(2~{R},4~{S})-2-[(1~{R})-2-(azepan-1-yl)-1-formamido-2-oxidanylidene-ethyl]-5,5-dimethyl-1,3-thiazolidine-4-carboxylic acid | C15 H25 N3 O4 S | 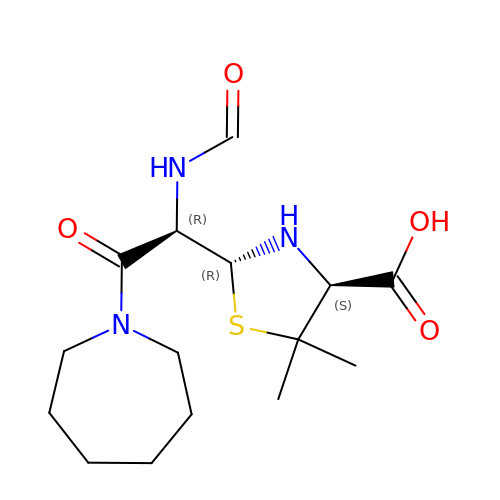PMJUGUXXJDBOJL-SDDRHHMPSA-N> SGGLDRGLIAVGMGLAVGLAALGTGVAQARIGAAGVGAIAEDRSNFGTALIFLLLPET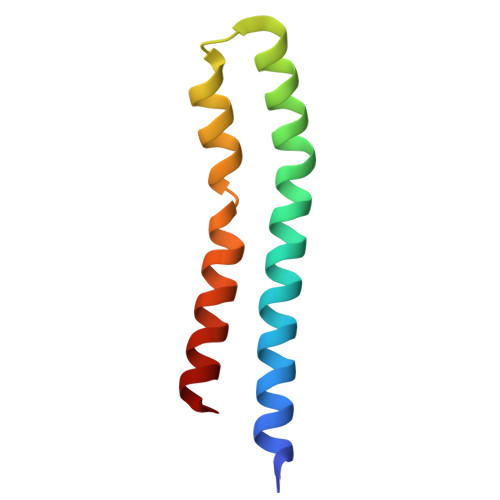LVIFGLLIAFILNGRL>HAMVSNAETETEKEQEEAAAASEELPVMPWATSVASGYTLLRDPHHNKGLAFTEEERDGHYLRGLLPPAVLSQELQIKKFMNTLRQYQTPLQRYIAMMNLQETDERLFYKLLIDNVVELLPFVYTPTVGEACQKYGSIFGRPQGLYVSLKDKGKVLEVLRNWPHRNIQVICVTDGERILGLGDLGCQGMGIPVGKLALYTALGGVDPSVCLPITIDVGTNNEKLLNDEFYIGLRQKRATGEEYDELIEEFMSAVKQFYGEKVLIQFEDFANHNAFDLLEKYSKSHLVFNDDIQGTASVVLAGLLAALKMVGGTLAEQTYLFLGAGEAGTGIAELIALEISKQTNAPIEECRKKVWLVDSKGLIVDSRKGSLQPFKKPWAHEHEPLKTLYDAVQSIKPTVLIGTSGVGRTFTKEIIEAMSSFNERPIIFSLSNPTSHSECTAEQAYTWSQGRSIFASGSPFAPVEYEGKTFVPGQSNNAYIFPGLGLGLVISGAVRVHEDMLLAASKALADQATQDNFEKGSIFPPFTSIRKISAHIAAAVAAKAYELG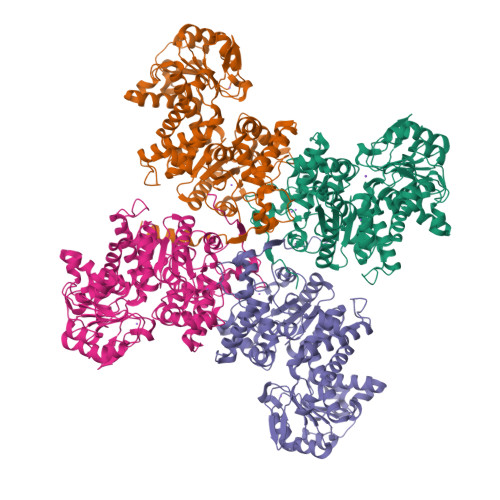LATRLPPPSDLVKYAENCMYTPVYRNYR[4x]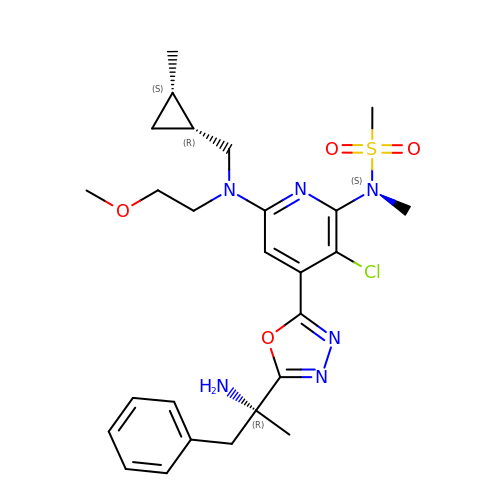(2R)-2-(5-{3-chloro-6-((2-methoxyethyl){[(1S,2S)-2-methylcyclopropyl]methyl}amino)-2-[methyl(methylsulfonyl)amino]pyridin-4-yl}-1,3,4-oxadiazol-2-yl)-1-phenylpropan-2-amine | C26 H35 Cl N6 O4 S | NIFMMESJJLKLHP-BNJIMDBKSA-N>SDCYFGNGSAYRGTHSLTESGASCLPWNSMILIGKVYTAQNPSAQALGLGKHNYCRNPDGDAKPWC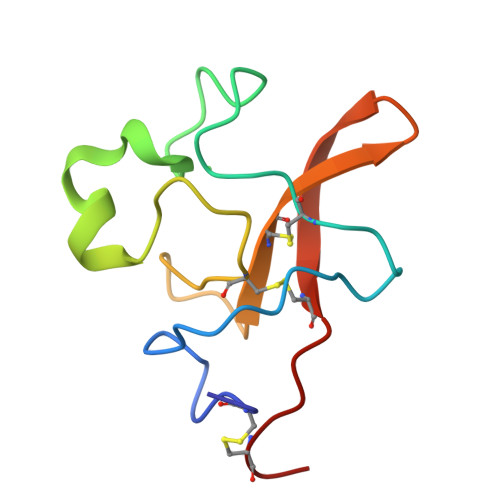HVLKNRRLTWEYCDVPSCST[3x]> GPDSMTSENPDVLLSRVINVVRAASSLASQDVDFYKNLDRGFSKDLKSKADKL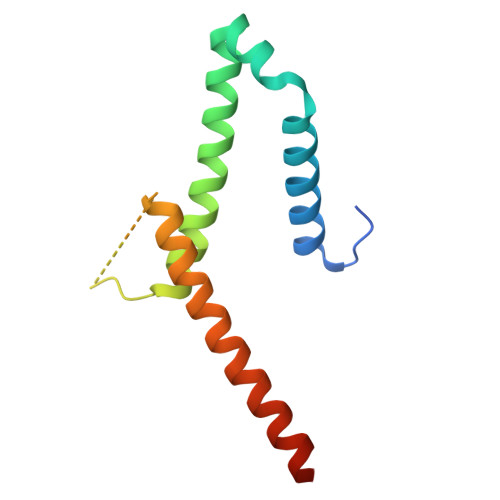ADMANEIILSIDEHHESFELKEEDISDLWNNFGNIMDNLLEMSDHSLDKLNCAINSKSRGSD>MSLERLRVAAYCRVSTDSEDQLNSYKSQVQYYTDMIKKNKEWVLADIYADEAITGTQVTKREDFQRMIN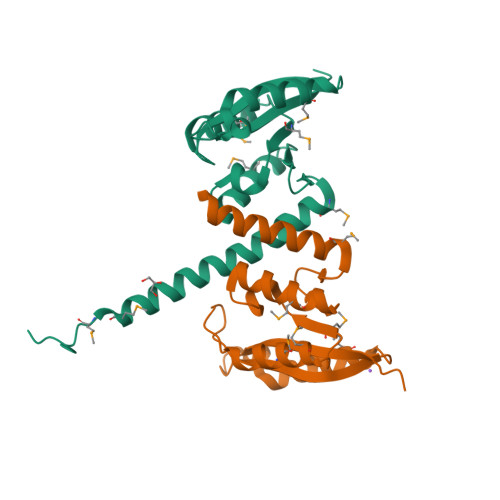DCMNGEIDMVFTKSISRFARNTLDTLKYVRMLKERNIAVYFEDEKINTLTMDGELLLVVLSSVAQQEVENISANVKKGLKMKMKRGELVGFQEGHHHHHH[2x]(2S)-2-{[1-(2-chlorophenyl)-1H-pyrazolo[3,4-d]pyrimidin-4-yl]oxy}-N-(5-chloropyridin-2-yl)-3-(2-hydroxyethoxy)propanamide | C21 H18 Cl2 N6 O4 | 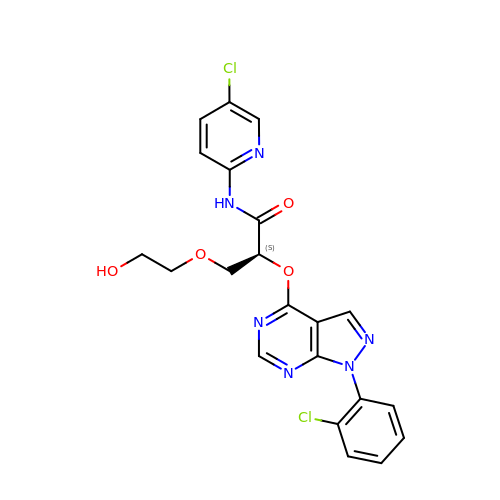KTWRHJPPIZQGRW-KRWDZBQOSA-N> MRGSHHHHHHGLVPRGSMQNPRTVSDTKRAFYAAHTRPIHSIYRRFIEELLVEIHLLRVNVDFRYSPLFALGVVTAFDQFMEGYQPEGDRDRIFHALCVAEEMNPQQLKEDAASWQQYQGRPLSQILDELNSGQPSAPLNSLNHTGKYSRLHAVGLYAFLQELAGEVTIHLNETLDQLAPVIPLPIEKVKRDLELYRSNLDKINQARSLMK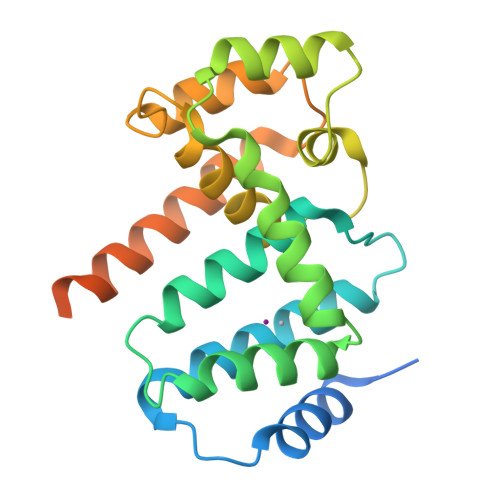ELVEQERKRRAQQTSAPPAVDASSDAPA> MPQLHYVPYDTPVEDVMRILKESGTLVIRNFLDQNTVQKVQDEVDDYVRNWNPGPGSKTKQPSNLSLMSKTYRCEVLNHPWMHAICERMFGPTYGDYWFNGGSILHLEPGENTQPIHQDHVFYQISKWRRPTDPDLTINFTMALTEFTVENGGTRVCPGSHLWENGHASPAEEDMVPVLMQPGDALILPGSMWHSAGANRTSEYRRGFATSF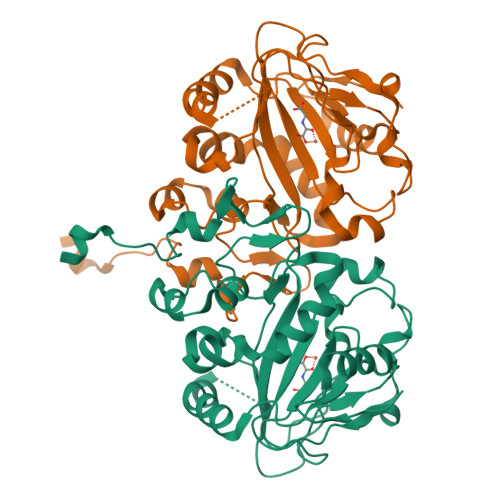HPCHFTPIESHHHLPREMVEEMTPLVQKMLGFRTLNLHNNVKVWKAGEGNLEDATGLKSVAAKLAAALEHHHHHH> MTVTRRHFLKLSAGAAVAGAFTGLGLSLAPTVARAELQKLQWAKQTTSICCYCAVGCGLIVHTAKDGQGRAVNVEGDPDHPINEGSLCPKGASIFQLGENDQRGTQPLYRAPFSDTWKPVTWDFALTEIAKRIKKTRDASFTEKNAAGDLVNRTEAIASFGSAAMDNEECWAYGNILRSLGLVYIEHQARIUHSPTVPALAESFGR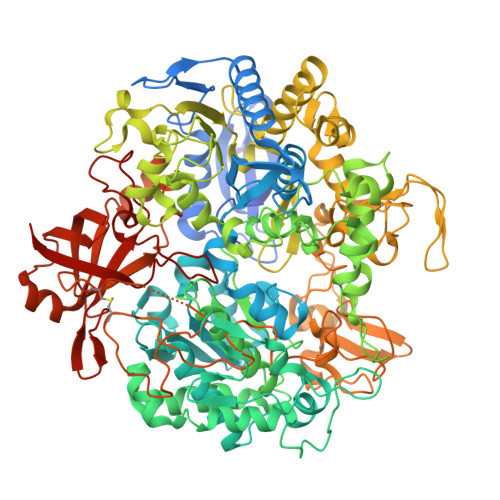GAMTNHWNDLANSDCILIMGSNAAENHPIAFKWVLRAKDKGATLIHVDPRFTRTSARCDVYAPIRSGADIPFLGGLIKYILDNKLYFTDYVREYTNASLIVGEKFSFKDGLFSGYDAANKKYDKSMWAFELDANGVPKRDPALKHPRCVINLLKKHYERYNLDKVAAITGTSKEQLQQVYKAYAATGKPDKAGTIMYAMGWTQHSVGVQNIRAMAMIQLLLGNIGVAGGGVNALRGESNVQGSTDQGLLAHIWPGYNPVPNSKAATLELYNAATPQSKDPMSVNWWQNRPKYVASYLKALYPDEEPAAAYDYLPRIDAGRKLTDYFWLNIFEKMDKGEFKGLFAWGMNPACGGANANKNRKAMGKLEWLVNVNLFENETSSFWKGPGMNPAEIGTEVFFLPCCVSIEKEGSVANSGRWMQWRYRGPKPYAETKPDGDIMLDMFKKVRELYAKEGGAYPAPIAKLNIADWEEHNEFSPTKVAKLMNGYFLKDTEVGGKQFKKGQQVPSFAFLTADGSTCSGNWLHAGSFTDAGNLMARRDKTQTPEQARIGLFPNWSFCWPVNRRILYNRASVDKTGKPWNPAKAVIEWKDGKWVGDVVDGGGDPGTKHPFIMQTHGFGALYGPGREEGPFPEHYEPLECPVSKNPFSKQLHNPVAFQIEGEKKAVCDPRYPFIGTTYRVTEHWQTGLMTRRCAWLVEAEPQIFCEISKELAKLRGIGNGDTVKVSSLRGALEAVAIVTERIRPFKIEGVDVHMVGLPWHYGWMVPKNGGDTANLLTPSAGDPNTGIPETKAFMVDVRKVWSHPQFEK> MQVLHVSSEMFPLLKTGGLADVIGALPAAQIADGVDARVLLPAFPDIRRGVTDAQV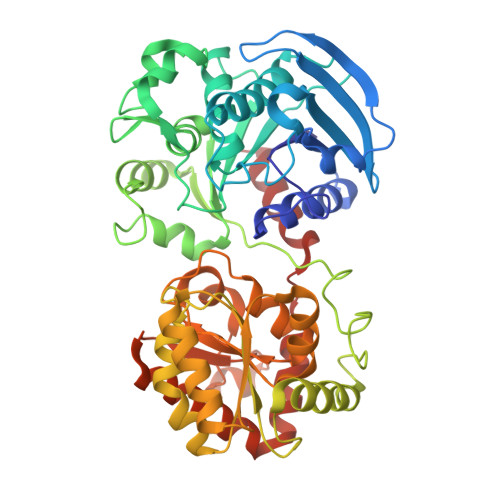VSRRDTFAGHITLLFGHYNGVGIYLIDAPHLYDRPGSPYHDTNLFAYTDNVLRFALLGWVGAEMASGLDPFWRPDVVHAHDWHAGLAPAYLAARGRPAKSVFTVHNLAYQGMFYAHHMNDIQLPWSFFNIHGLEFNGQISFLKAGLYYADHITAVSPTYAREITEPQFAYGMEGLLQQRHREGRLSGVLNGVDEKIWSPETDLLLASRYTRDTLEDKAENKRQLQIAMGLKVDDKVPLFAVVSRLTSQKGLDLVLEALPGLLEQGGQLALLGAGDPVLQEGFLAAAAEYPGQVGVQIGYHEAFSHRIMGGADVILVPSRFEPCGLTQLYGLKYGTLPLVRRTGGLADTVSDSSLENLADGVASGFVFEDSNAWSLLRAIRRAFVLWSRPSLWRFVQRQAMAMDFSWQVAAKSYRELYYRLK> SYQSTCGLRQYSQRQRR;> IKGGLFADIASHPWQAAIFAKHRRSPGERFLCGGILISSCWILSAAHCFQERFPPHHLTVILGRTYRVVPGEEEQKFEVEKYIVHKEFDDDTYDNDIALLQLKSDSSRCAQESSVVRTVCLPPADLQLPDWTECELSGYGKHEALSPFYSERLKEAHVRLYPSSRCTSQHLLNRT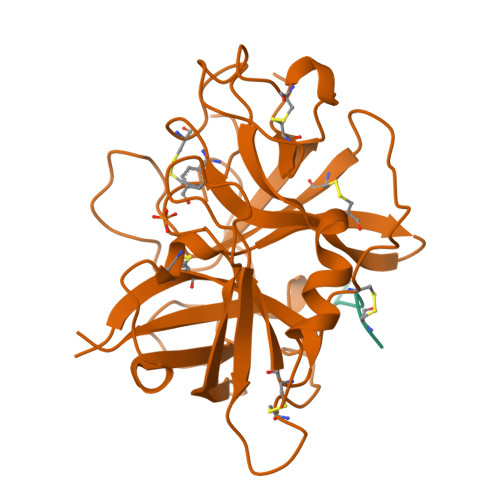VTDNMLCAGDTRSGGPQANLHDACQGDSGGPLVCLNDGRMTLVGIISWGLGCGQKDVPGVYTKVTNYLDWIRDNMRP>CCIIICCCGG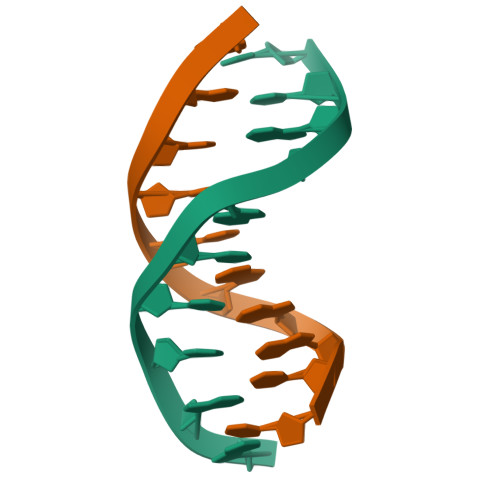[2x]>MVRRRGGKTAGSKRPKMSSKNFGANRKRDFRRPARKSKAKKARSMAPAKTVRKSTTAGAHSKHFSVIGNPFSKATQQPQIPDGRMLESLPRRCQLVTEIRNNVTVGSNPTYILVAPSLGLAFQAYQDTNVPGGLDSSVYGLQNRGCTVRANLSATSIENYNDIAKWRIVSQGINLKLNNVEDENDGWYEACRFQHDWTPDELCLRSTENDASTISQDEDLVMGVISSSFMNGALNTIGNNMVEQRGYESGLLKNIHKRMFQLHNNTSAIRPKTLQGQFNYGSEITFSGTESEARFTDVPSNRQLVDSLWHNDYDCILIKLYPRENTGAA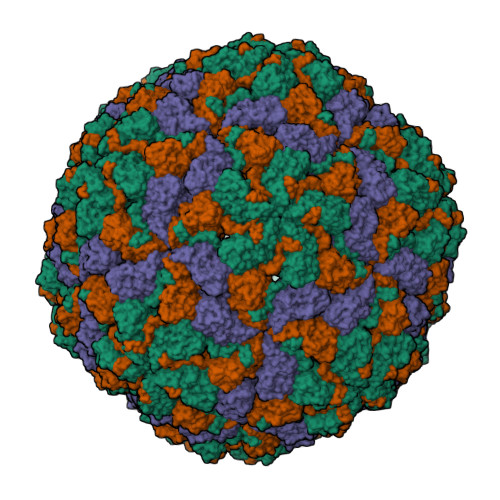GQTGSALIVNAIQNLELQYSPTSDLSTYHIANKRARMVEAKLDKKNNTDAAGEPFVPGSSR[3x]> GSHMGGERTVTIRRQTVGGFGLSIKGGAEHNIPVVVSKISKEQRAELSGLLFIGDAILQINGINVRKCRHEEVVQVLRNAGEEVTLTVSFLKRAPGSAYGSVKAYTNFDAERDALNIETAIKTKGVDEVTIVNILTNRSNEQRQDIAFAYQRRTKKELASALKSALSGHLETVILGLLKTPAQYDASELKASMKGLGTDEDSLIEIICSRTNQELQEINRVYKEMYKTDLEKD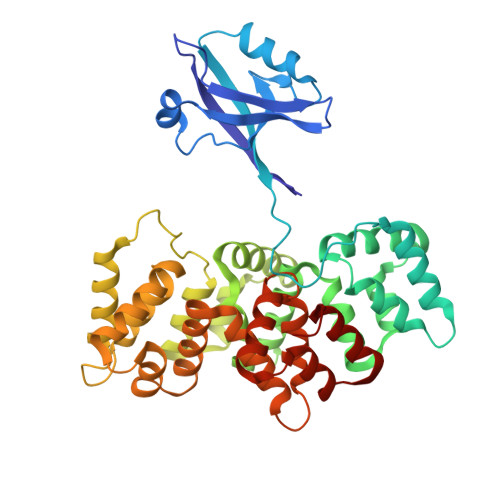IISDTSGDFRKLMVALAKGRRAEDGSVIDYELIDQDARDLYDAGVKRKGTDVPKWISIMTERSVPHLQKVFDRYKSYSPYDMLESIRKEVKGDLENAFLNLVQCIQNKPLYFADRLYDSMKGKGTRDKVLIRIMVSRSEVDMLKIRSEFKRKYGKSLYYYIQQDTKGDYQKALLYLCGGDD>[2x]MPIITDVYAREVLDSRGNPTVEVEVLTESGAFGRALVPSGASTGEHEAVELRDGDKSRYLGKGVTKAVENVNEIIAPEIIEGEFSVLDQVSIDKMMIALDGTPNKGKLGANAILGVSIAVARAAADLLGQPLYKYLGGFNGKQLPVPMMNIVNGGSHSDAPIAFQEFM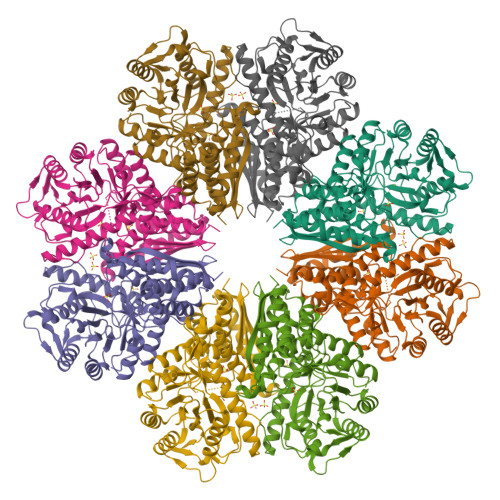ILPVGATTFKESLRWGTEIFHNLKSILSKRGLETAVGDEGGFAPKFEGTEDAVETIIQAIEAAGYKPGEEVFLGFDCASSEFYENGVYDYSKFEGEHGAKRTAAEQVDYLEQLVDKYPIITIEDGMDENDWDGWKQLTERIGDRVQLVGDDLFVTNTEILAKGIENGIGNSILIKVNQIGTLTETFDAIEMAQKAGYTAVVSHRSGETEDTTIADIAVATNAGQIKTGSLSRTDRIAKYNQLLRIEDELFETAKYDGIKSFYNLDKLEHHHHHH>MRTRSTISTPNGITWYYEQEGTGPDIVLVPDGLGECQMFDSSVSQIAAQGFRVTTFDMPGMSRSAKAPAETYTEVTAQKLASYVISILDALDIKHATVWGCSSGASTVVALLLGYPDRIRNAMCHELPTKLLDHLSNTAVLEDEEISNILANVMLNDVSGGSEAWQALGVEVHARLHKNYPVWARGYPRTIPPSAPVQDVEALRGKPLDWTVGAATPTESFFDNIVTATKAGVNIGLLPGMAFPYV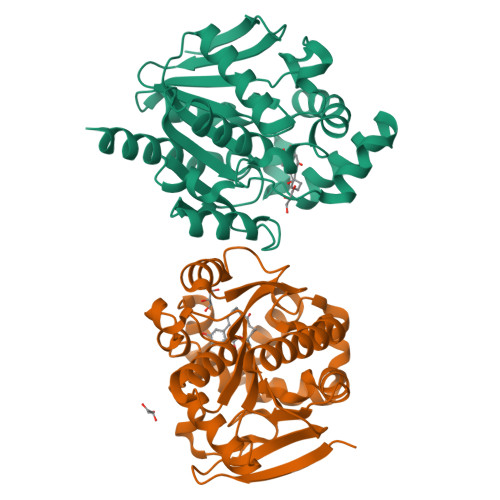SHPDVFAKYVVETTQKHLWNSSSVDKLAAALEHHHHHH[2x]>AEFVFEWFGSNESGAEFGTNIPGVWGTDYIFPDPSAISTLIDKGMNFFRVQFMMERLLPDSMTGSYDEEYLANLTTV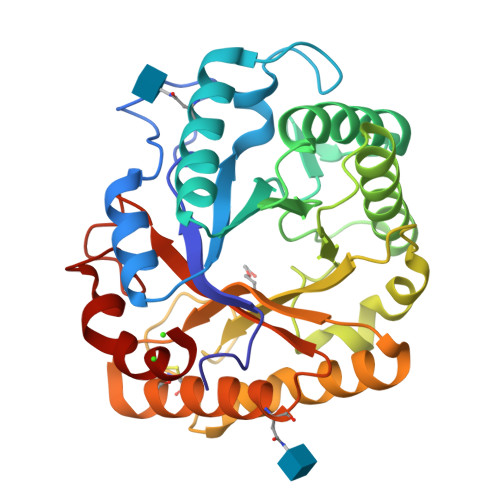IKAVTDGGAHALVDPHNYGRYNGEIISSTSDFQTFWENLAGQYKDNDLVMFDTNNEYHDMDQDLVLNLNQAAINGIRAAGATSQYIFVEGNSWTGAWTWVDVNDNMKNLTDPEDKIVYEMHQYLDSDGSGTSETCVSETIGKERVTEATQWLKDNKKVGFIGAYAGGSNDVCRSAVSGMLEYMANNTDVWKGASWWAAGPWWGDYIFSLEPPDGTAYTGMLDILEAYL[2x]Plasminogen activator inhibitor-1 (PAI-1), a member of the serine protease inhibitor (serpin) superfamily, acts by inhibiting tissue-type (tPA) and urokinase-type (uPA) plasminogen activators (PAs). To this end, PAI-1 exposes a flexible reactive center loop (RCL) at its surface, which contains the substrate-mimicking peptide sequence Arg346-Met347 (designated as P1–P1′). In contrast to other serpins, PAI-1 has the unique ability to spontaneously convert into a stable latent form by inserting the RCL segment N-terminal to the P1–P1′ cleavage site (residues 331 to 346, designated as P16-P1) in the core β-sheet A without prior cleavage to become strand 4 (s4A). Structural analysis of PAI-1 crystals soaked with a solution containing TM5484 allowed us to unambiguously identify its binding site similar to the Vn-binding region comprising hE, hF, and s1A.

After crystallization screening of two stabilized active PAI-1 mutants, PAI-1-W175F and PAI-1-N150H-K154T-Q301P-Q319L-M354I (PAI-1-stab), free or in complex with PAI-1 neutralizing nanobodies (Nb42 and Nb64), diffracting crystals were obtained and soaked with the compounds. In the case of the PAI-1-stab crystal, two PAI-1 molecules (chains A and B) were observed of which only one had TM5484 compound bound (chain A). Indeed, in the case of the second PAI-1 molecule (chain B), access to the binding site is restricted due to close crystallographic contacts with a PAI-1 molecule from the neighboring ASU. Comparison of TM5484 in the compound-bound structures shows TM5484 at the crystallographic interface between PAI-1 and Nb64 (in the PAI-1/Nb42/Nb64 crystal), or between two PAI-1 molecules (in the PAI-1-stab crystal). Comparison of the TM5485-bound PAI-1/Nb42/Nb64 and PAI-1-stab structures revealed that the TM5484 molecule bound in two different orientations, hereafter referred to as “orientation 1” and “orientation 2”. In this respect, it is notable that the carboxylic acid interacts with PAI-1 Lys122 (s1A) through the formation of a salt bridge independent of the orientation of TM5484, and with PAI-1 Thr120 (s1A) through an additional hydrogen bond in orientation 2. In orientation 2, the Cl-atom is located 4.3 Å away from the sidechain of Trp139 in hF and 5.4 Å away from the ring centroid in an edge-on geometry, thus resulting in weaker interactions. Additionally, the Cl-atom makes a 3.4 Å van der Waals interaction with the side chain of Ile135 in hF. In orientation 2, however, the neighboring PAI-1-stab molecule forms a π–π stacking interaction and an electrostatic π-anion interaction with the chloroanthranilic acid moiety of TM5484 through Trp86. Furthermore, Lys88 and Val334 engage in hydrophobic interactions (π-alkyl and amide-π stacking, and π-sigma, respectively) with the phenylfuran moiety of TM5484.

>[2x]VHHPPSYVAHLASDFGVRVFQQVAQASKDRNVVFSPYGVASVLAMLQLTTGGETQQQIQAAMGFKIDDKGMAPALRHLYKELMGPWNKDEISTTDAIFVQRDLKLVQGFMPHFFRLFRSTVKQVDFSEVERARFIINDWVKTHTKGMISHLLGTGAVDQLTRLVLVNALYFNGQWKTPFPDSSTHRRLFHKSDGSTVSVPMMAQTNKFNYTEFTTPDGHYYDILELPYHGDTLSMFIAAPYEKEVPLSALTNILSAQLISHWKGNMTRLPRLLVLPKFSLETEVDLRKPLENLGMTDMFRPFQADFTSLSDQEPLHVALALQKVKIEVNESGTVASSSTAVIVSARMAPEEIIIDRPFLFVVRHNPTGTVLFMGQVMEP1,4-DIDEOXY-1,4-[[2R,3R)-2,4-DIHYDROXY-3-(SULFOXY)BUTYL]EPISULFONIUMYLIDENE]-D-ARABINITOL 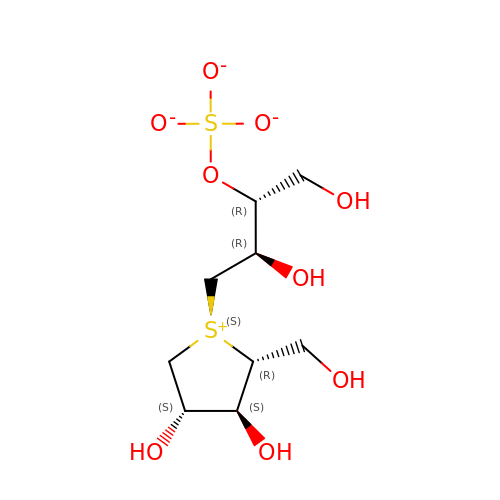INNER SALT | C9 H18 O9 S2 | NYHLFUZUGSMDBR-ITGKUZSGSA-L>[2x]MTVVPVTSADLDAAEVSWFSALCSDDYAYLGVPDGSLRSSFEHCSDIVKKAEELGFRNILCPSSYQVGQDTLSFVAGCAPISDRINFLAAIRCGEMQPIMLARTVATLDHMLKGRLTLNVISSDFPGEVADSAFRYKRSHEVVEILRQAWTRDTIDHDGEIYQFKGVSTEPARPYQLNGGPLLYFGGYSPDALE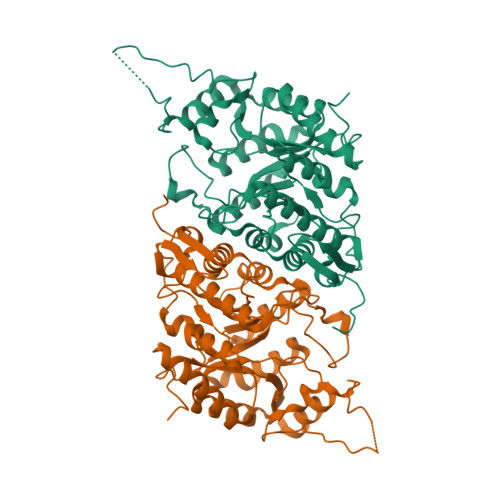LCGAQCDVYLMWPETKDQLADRMRAAHERAAAHGRTLDYGLRVHMVVRDTEQEAREYADHLVSKLDDEYGQLIRNRAHDSGSLGVSHQARARELADKFGYVEPNLWTGIGRARSGCGAALVGSTDQVLSALEEYQKMGIRAFILSGYPHLDEAEHFGTKVLPQMKTCSLPHAYGRVPSETPATPLGNGERHLEHHHHHH> XDPAWYEC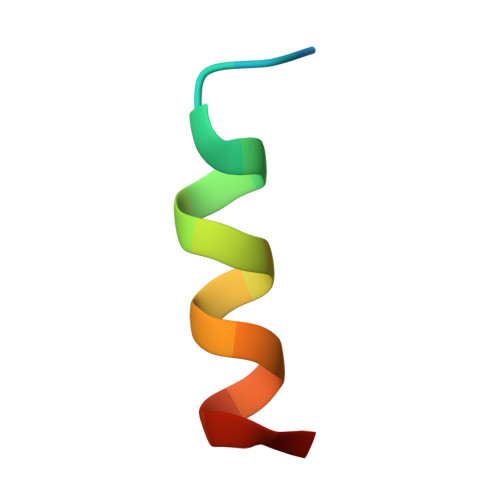LEAALLCQQVX>CGGGE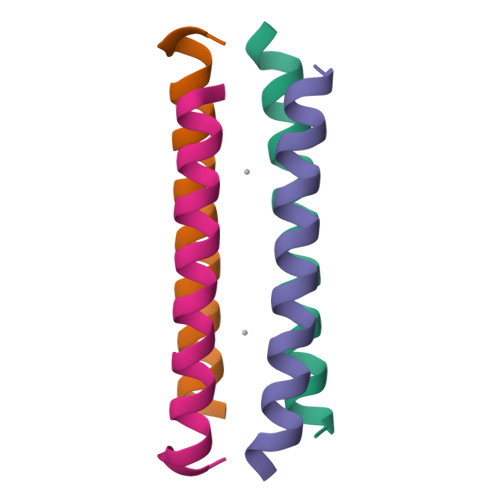IWKLHEEFLKKFEELLKLHEERLKKMX[4x]>MLSLTRILRKKIPVHELAGKISRPPLRPFSVVVASDEKGGIGDGGTIPWEIPEDMQYFRRVTTNLRGKNVKPSPSKRNAVVMGRKTWDSLPPKFRPLSNRLNVVLSRSATKEQLLAGIPDPIKRAEAANDVVAVNGGLEDALRMLVSKEHTSSIETVFCIGGGTIYKQALCAPCVNVLQAIHRTVVRPASNSCSVFFDIPAAGTKTPEGLELVRES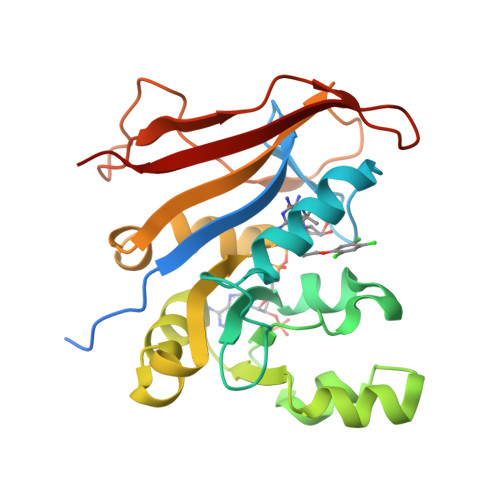ITDERVSTGAGGKKYQFEKLVPRN[2x]> MGSMATLKAQHLAKSYKG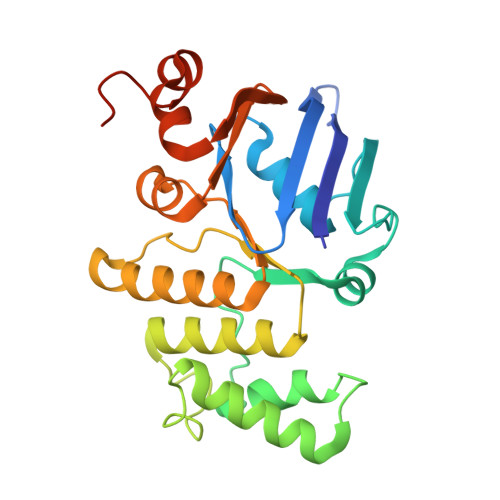RQVVRDVSMSIDSGQIVGLLGPNGAGKTTCFYMIVGLVQADQGVVRIDEQNVTHLPMHGRARAGIGYLPQEASIFRKLSVSDNIMAILETRSDLDRNGRKEALEGLLQEFHIHHIRDNLGMSLSGGERRRVEIARALASAPKFILLDEPFAGVDPISVGDIKQIIHHLKAKGIGILITDHNVRETLDICETAYIVNDGQLIAEGDAESILANDLVKEVYLGHEFRLKLHHHHHH A 13-member family of ABA receptors PYR/PYL/RCAR (PYLs) in Arabidopsis thaliana was genetically and biochemically identified. Upon binding (+)-ABA, dimeric PYLs underwent a pronounced conformational rearrangement, and then bound and inhibited the group A protein phosphatases type 2Cs (PP2C), including ABI1, ABI2, HAB1 and PP2CA. PYLs/PP2C heterodimer blocked substrates binding to PP2Cs, and thus released downstream transcription factors SnRK2 kinases formerly inhibited by PP2C. Structural analysis along with biochemical data in vitro demonstrated that steric hindrance and hydrophobic interaction in the pocket of PYLs were crucial for their stereospecificity to ABA enantiomers.

The complex of PYL9 with (+)-ABA was solved at 2.68 Å resolution. Each asymmetric unit contained a symmetric cis-dimer. One protomer had four α-helices and seven β-sheets, sharing the similar arrangements of other known PYLs. Loops L4 and L5 played the role of the gate and the latch respectively, which locked the (+)-ABA in a conserved pocket. The (+)-ABA was encaged in the cavity by abundant hydrophobic interactions, several hydrogen bonds and two salt bridges. Surprisingly, a disulphide bond between C34 and C159 was observed in PYL9-(+)-ABA structure. On the other hand, the pocket ingeniously arranged a bigger room to accommodate the 8′, 9′ dimethyl of (+)-ABA, for example, the bulky residue I112 of PYL9 was involved in direct binding 8′ methyl group of (+)-ABA, respectively. However, due to the confinement of 9′ methyl group by the coordination of several bulk residues on the entrance of the pocket of PYLs, the 7′ and 8′ methyl groups of (−)-ABA were uncomfortable with the bulk side chains, such as I112 and L165 of PYL9, which make (−)-ABA incompatible in the pocket for the strong steric constraints. By contrast, PYL9 did not inhibit PP2C activity at 10 µM or even higher concentration of (−)-ABA.

>MGSSHHHHHSSGENLYFQMMDGVEGGTAMYGGLETVQYVRTHHQHLCRENQCTSALVKHIKAPLHLVWSLVRRFDQPQKYKPFVSRCTVIGDPEIGSLREVNVKSGLPATTSTERLELLDDEEHILGIKIIGGDHRLKNYSSILTVHPEIIEGRAGTMVIESFVVDVPQGNTKDETCYFVEALIRCNLKSLADVSERLASQDITQ[2x]>[6x]MRGSHHHHHHGSTTF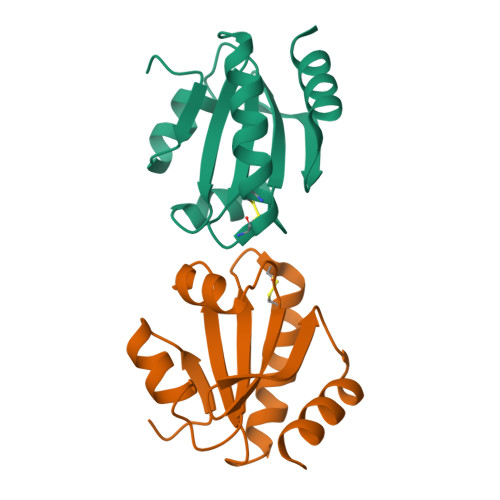NIQDGPDFQDRVVNSETPVVVDFHAQWCGPCKILGPRLEKMVAKQHGKVVMAKVDIDDHTDLAIEYEVSAVPTVLAMKNGDVVDKFVGIKDEDQLEAFLKKLIG>GQDMVSPPPPIADEPLTVNTGIYLIECYSLDDKAETFKVNAFLSLSWKDRRLAFDPVRSGVRVKTYEPEAIWIPEIRFVNVENARDADVVDISVSPDGTVQYLERFSARVLSPLDFRRYPFDSQTLHIYLIVRSVDTRNIVLAVDLEKVGKNDDVFLTGWDIESFTAVVKPANFALEDRLESKLDYQLRISRQYFSYIPNIILPMLFILFISWTAFWSTSYEANVTLVVSTLIAHIAFNILVETNLPKTPYMTYTGAIIFMIYLFYFVAVIEVTVQQYLKVESQPARAASITRASRIAFPVVFLLANIILAFLFFGF[5x]

At present, the best structurally characterized pLGIC is the G. violaceus ligand-gated ion channel (GLIC), of prokaryotic origin. Each subunit consists of an extracellular domain (ECD), predominantly in a β-sandwich fold, and a transmembrane domain (TMD) composed of four helices, labeled M1–M4. However, the GLIC is a pH-gated channel, activated by lowering the pH, with a maximal activation at pH 4 and a pH50 around 5. We instead found that proton activation is a complex multiple loci mechanism, with the key contribution stemming from the coupling interface between the extracellular and transmembrane domain, with E35 acting as a key proton-sensing residue.

Among the other titratable residues of the TMD, neither a mutation of E272Q nor E282Q produced an overall significant effect, albeit a significant negative ΔpH50 was observed for E272Q, which was previously reported to be nonfunctional when mutated to A. In contrast, the mutation of either E222 or E243 as Q or A, as well as H277Q, all produced significant loss-of-function effects, pointing to the key role of these residues in activation. Mutation of H277, which lies in the adjacent M3 α-helix (nearby E222) with possible electrostatic interaction, has also previously been shown, using noncanonical amino acid substitution to decrease the pH50. The structure of H277Q was performed and was also found to have no apparent deviation from the apparently open pH 4 conformation, which further corroborates the several previously published works that show H277 does not appear to play a role in proton gating. Mutations at both entrances of the ion channel, E243 (outer ring) and E222/H277 (inner rings), as well as at the middle of the TMD within each subunit four-helix bundle (H235), produced significant decreases in proton sensitivity, but again here, the pattern of phenotypes does not allow discriminating between proton sensing and gating. E222/H277 might also contribute to pH sensing, implying in this case the diffusion of protons from the extracellular compartment, possibly through the ion channel itself. The E222/H277 pair most likely confers the intracellular proton concentration sensitivity of the GLIC, which was reported from inside-out patch clamp experiments. The functional results indicate either a sensitivity to protons or a structural importance for both H235 and H277, neither of which are crucial for proton-elicited gating of the GLIC.> MELPKEMEEYFEMLQREIDKAYEIAKKARAQGKDPSLDVEIPQATDMAGRVESLVGPPGVAKRIRELVKEYGKEIAALKIVDEIIEGKFGDLGSREKYAEQAVRTALAILTEGIVSAPIEGIANVKIKRNTWADNSEYLALYYAGPIRSSGGTAQALSVLVGDYVRRKLGLDRFKPSEKHIERMVEEVDLYHRAVTRLQYHPSPEEVRLAMRNIPIEITGEATDDVEVSHRDVPGVETNQLRGGAILVLAEGVLQKAKKLVKYIDKMGIEGWEWLKEFVEAKEKGEPKEEGKEESLAESTLEETKVEVDMGFYYSLYQKFKEEIAPSDKYAKEVIGGRPLFSDPSKPGGFRLRYGRSRASGFATWGINPATMILVDEFLAIGTQLKTERPGKGAVVTPVTTIEGPIVKLKDGSVLRVDDYNLALKVREDVEEILYLGDAVIAFGDFVENNQTLLPANYCEEWWILEFVKALKEIYEVHLEPFTENEEESIEEASDYLEIDPEFLKEMLRDPLRVKPPVELAIHFSEVLGIPLHPYYTLYWNSVEPKDVEKLWRLLKNYAEIEWSNFRGIKFAKKIVISQEKLGDSKRTLELLGLPHTVRDGNVIVDYPWAAALLTPLGNLNWEFMAKPLYATIDIINENNEIKLRDRGISWIGARMGRPEKAKERKMKPPVQVLFPIGLAGGSSRDIKKAAEEGKVAEVEIAFFKCPKCGHVGPEHLCPNCGTRKELLWVCPRCNAEYPESQAEGYNYTCPKCNVKLRPYAKRKIRPSELLNRAMENVKVYGVDKLKGVMGMTSGWKMPEPLEKGLLRAKNDVYVFKDGTIRFDATDAPITHFRPREIGVSVEKLRELGYTHDFEGKPLVSEDQIVELKPQDIILSKEAGRYLLKVAKFVDDLLEKFYGLPRFYNAEKMEDLIGHLVIGLAPHTSAGIVGRIIGFVDALVGYAHPYFHAAKRRNCDGDEDAVMLLLDALLNFSRYYLPEKRGGKMDAPLVITTRLDPREVDSEVHNMDIVRYY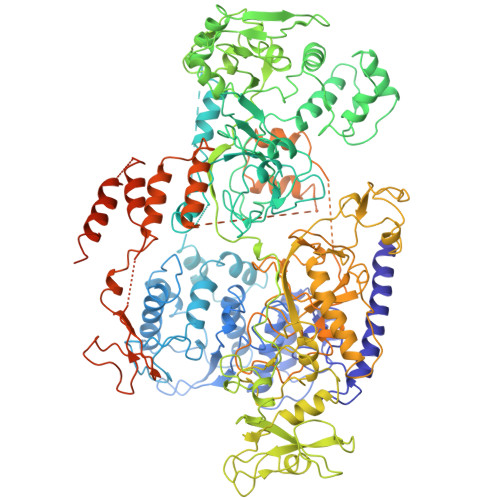PLEFYEATYELKSPKELVGVIERVEDRLGKPEMYYGLKFTHDTDDIALGPKMSLYKQLGDMEEKVRRQLEVAKRIRAVDEHGVAEKILNSHLIPDLRGNLRSFTRQEFRCVKCNTKFRRPPLNGKCPVCGGKIVLTVSKGAIEKYLGTAKMLVTEYNVKNYTRQRICLTERDIDSLFENVFPETQLTLIVNPNDICQRLVMARTGEVNKSGLLENLSNGSKKTEKAEKAEKPRKKSDEKPKKKRVISLEEFFSRKSK>MVIQVTNKEEFEAILSEADKLVVVDFFATWCGPCKMIAPFFEELSEEYPDKVVFIKVDVDEVPDVAAKYGIT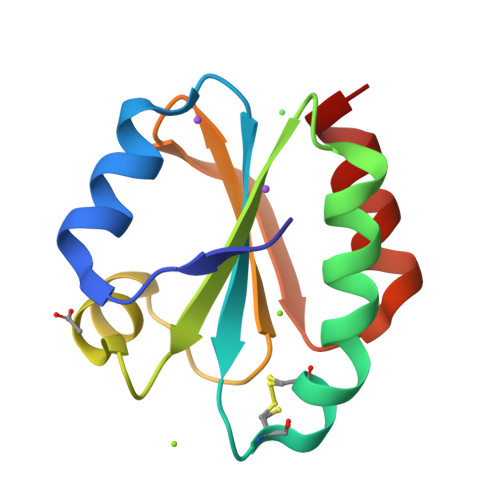SMPTFKFFKNGKKVDELVGANQEKLKQMILKHAP[2x]> MTIRSYKNLNLVRANIETESRQFIENKNYSIQSIGPMPGSRAGLRVVFTRPGVNLATVDIFYNGDGSTTIQYLTGANRSLGQELADHLFETINPAEFEQVNMVLQGFVETSVLPVLELSADESHIEFREHSRNAHTVVWKIISTSYQDELTVSLHITTGKLQIQGRPLSCYRVFTFNLAALLDLQGLEKVLIRQEDGKANIVQQEVARTYLQTVMADAYPHLHVTAEKLLVSGLCVKLAAPDLPDYCMLLYPELRTIEGVLKSKMSGLGMPVQQPAGFGTYFDKPAAHYILKPQFAATLRPEQINIISTAYTFFNVERHSLFH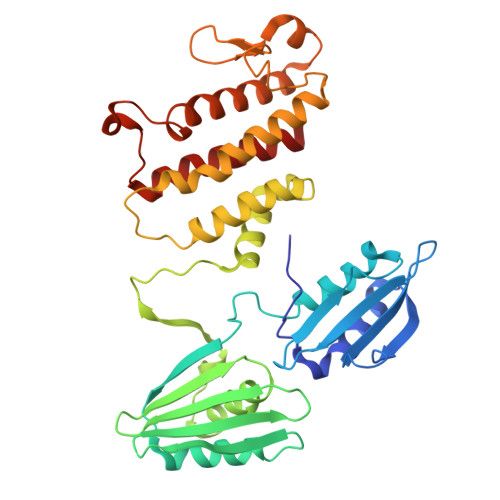METVVDASRMISDMARLMGKATRAWGIIKDLYIV>MSLHACRMKLITAIVKPFTLTDIKDALEQAGVQGMTVTETQGFGQQKGHTEVYRGAEYAVDFVPKVKIEVIISDAQAEEVINIIVETARTGKVGDGKVWMTNIEELVRVRTGERGEAAL[3x]

PII proteins are ubiquitous signaling proteins that are involved in the regulation of the nitrogen/carbon balance in bacteria, archaea, and some plants and algae. Signal transduction via PII proteins is modulated by effector molecules and post-translational modifications in the PII T-loop. In the present study, crystal structures of the PII protein GlnK from Corynebacterium glutamicum have been determined, namely of adenylylated GlnK (adGlnK) and unmodified unadenylylated GlnK (unGlnK). The allosteric signal that links effector binding to the regulation of the activity of PII-interacting proteins is primarily transduced via the T-loop, which adopts different conformations depending on the nature and combination of bound effectors.

The protein crystallized in the tetragonal space group P43212 and the final model contains one GlnK trimer per asymmetric unit. The three subunits deviate from each other by an average r.m.s.d. value of 0.6 Å (Cα positions). Hence, and as is the case for other PII proteins, GlnK from C. glutamicum can be considered to be a permanent homotrimeric protein. Three phosphate molecules are bound to trimeric GlnK in unGlnK. All three phosphates bind highly similarly and interact exclusively with residues from the B- and C-loops. The phosphates form a direct hydrogen bond to the backbone of Gly87 from the B-loop, as well as additional hydrogen bonds to the side chains of Arg101 and Arg103, which either precede or are part of the C-loop.2-Thiouridine (s2U) is a nucleobase modification that confers enhanced efficiency and fidelity both on modern tRNA codon translation and on nonenzymatic and ribozyme-catalyzed RNA copying. We have discovered an unusual base pair between two 2-thiouridines that stabilizes an RNA duplex to a degree that is comparable to that of a native A:U base pair. High-resolution crystal structures indicate similar base-pairing geometry and stacking interactions in duplexes containing s2U:s2U compared to those with U:U pairs. Notably, the C=O···H–N hydrogen bond in the U:U pair is replaced with a C=S···H–N hydrogen bond in the s2U:s2U base pair.

The sequence UU1, 5′-AGA GUA GAUC UUC UCU-3′, can form a duplex with two U/U pairs at the positions of the underlined nucleotides. The UU1, UU2, and SS1 structures pack similarly, with one strand in each asymmetric unit forming a duplex with another strand in a different asymmetric unit. The U:U pair in UU1 forms a shorter hydrogen bond between N3 of U5 and O4 of U12′ compared to the bond between the O2 of U5 and N3 of U12′ (3.0 vs 3.4 Å). However, since a thiocarbonyl is a weaker H-bond acceptor, the strength of the H-bond in the C=S···H interaction could be slightly weaker than that in the C=O···H. Besides the similar H-bond lengths, all of the nucleotides are in the C3′-endo conformation in both structures. We found no significant perturbations between the geometric parameters of UU1 and SS1. We also calculated the overlap areas of the base pair steps in both sequences to explore the base stacking interactions. Only a 2.68 Å2 difference was observed on the total overlap areas of all base pair steps, which indicates that the s2U:s2U pair has a negligible impact on base stacking in the crystals.

> AGAGUAGAUCUUCUCU>[4x]HHHHHHSSGLVPRGSHMLLTADTVLTGTELLRPGWLEIASDRVVAVGAGAPPAQADRNLGAATVVPGFVDTHLHGGGGGNFSAATDDETARAVALHRAHGSTTLVASLVTAGPEDLLRQVSGLARQVRAGLIDGIHLEGPWLSTLRCGAHQPVLMRDPDPGEIGRVLDAGEGTVRMVTIAPERDGALAAIAQLVNAGVVAAVGHTEATYDQTRAAIDAGATVGTHLFNAMRPIDRREPGPAVALTEDSRVTVEMIVDGVHVAPAIYRHITQTVGPERLSLITDAMAATGMSDGVYRLGPLDIDVVAGVARVAGTDTIAGSTATMEQVFRLAVAHCGLPRDDALSLAVRQACVNPARALGLPAAGLAAGARADLVVLDHDLAVTAVMRAGEWVVTPGAAHTV

NagA enzymes (EC 3.5.1.25) are widespread in nature and found in a range of eukaryotic and prokaryotic species as metal-dependent enzymes with a physiological role in catalyzing the deacetylation of GlcNAc6P to yield GlcN6P and acetate. Our X-ray crystallographic structure determination reveals that MSNagA conforms to the urease structural superfamily, with the same overall fold, domain topology, and architecture as other NagA enzymes whose structures have been determined. Domain I (residues 52–344) is a twisted (β/α)8-TIM barrel that is comprised of eight alternating β-stands and α-helices and encloses the catalytic site of the enzyme and the metal-binding site. Domain II is a small β-barrel comprising eight β-strands contributed from the N and C termini of the MSNagA protein (amino acids 1–51 and 344–382).

The MSNagA protein in the absence of ligand crystallized in space group P1 with four molecules in the asymmetric unit. Although no divalent cations were added during the purification steps, well defined electron density corresponding to two bound metal ions was clearly visible in the cavity of the (α/β) barrel buried at the bottom of the active-site cleft. Each MSNagA monomer in both the ligand-free and ligand-bound models contains two metal ions positioned between 3.1 and 3.4 Å apart from each other. Given that the same protein expressed in M. smegmatis contains predominantly zinc, it was decided to model the metal-binding sites as zinc rather than iron (see “Experimental procedures”). In all chains of the apo-structure, the metal ion that is more buried (M1) makes four interactions coordinated by the side chains His-56, His-58, Glu-122, and Asp-267. The second metal ion (M2) is held in position by the side chains of residues His-188, Glu-122, and His-209. Coordination is completed by water molecules with one water molecule modeled as bridging both of the metals and another bound to M1. In both of the MSNagA crystal structures, the protein forms a homodimer burying a total of 3,200 Å2 of the surface area. The carbonyl group of the GlcNAc6P substrate is positioned ∼2.5 Å from the M1 metal ion, which is ideally primed to stabilize the transition state intermediate formed during catalysis. It is of interest to note, by comparison of the apo- and ligand-bound structures, that there is little conformational change in the binding pocket upon substrate binding to MSNagA.> AVPFVEDWDLVQTLGEGAYGEVQLAVNRVTE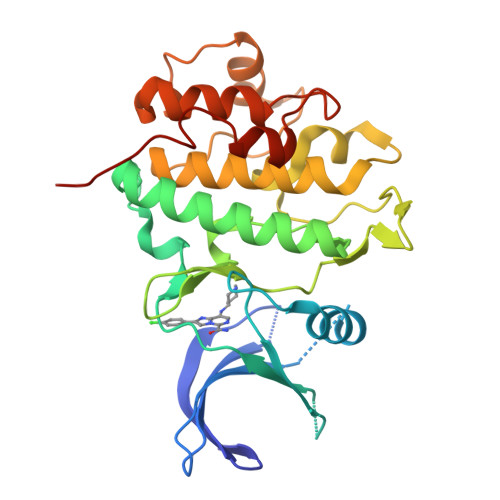EAVAVKIVDMKRAVDCPENIKKEICINKMLNHENVVKFYGHRREGNIQYLFLEYCSGGELFDRIEPDIGMPEPDAQRFFHQLMAGVVYLHGIGITHRDIKPENLLLDERDNLKISDFGLATVFRYNNRERLLNKMCGTLPYVAPELLKRREFHAEPVDVWSCGIVLTAMLAGELPWDQPSDSCQEYSDWKEKKTYLNPWKKIDSAPLALLHKILVENPSARITIPDIKKDRWYNKPLKKGAK>[2x]MSVSSIISHAQFDRMLLHRNDGACQAKGFYTYDAFVAAANAFPGFGATGS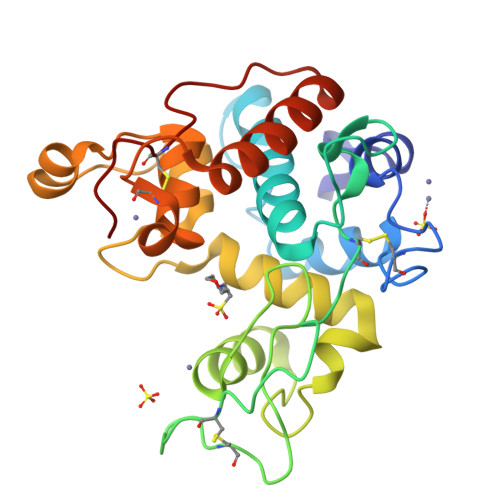TDARKRDVAAFLAQTSHETTGGWATAPDGAFAWGYCFKQERGAAADYCTPSAQWPCAPGKRYYGRGPIQLSHNYNYGPAGRAIGVDLLRNPDLVATDPTVSFKTALWFWMTAQAPKPSSHAVITGKWSPSGADRAAGRAPGFGVITNIINGGLECGHGQDSRVADRIGFYKRYCDILGVGYGDNLDCYNQRPFA7-[[4-chloranyl-3-(methylaminomethyl)phenoxy]methyl]quinolin-2-amine 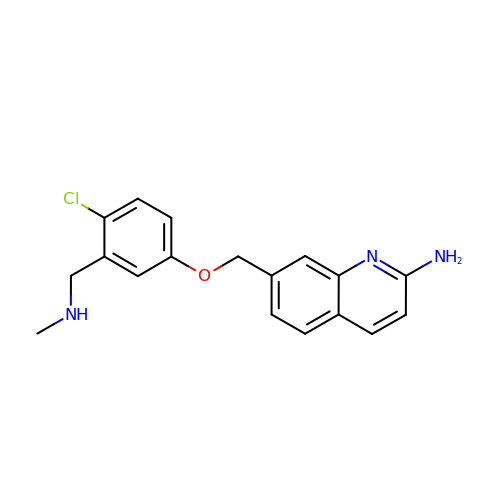| C18 H18 Cl N3 O | SVDORCPNIHFYFA-UHFFFAOYSA-N1-(3-PYRROLIDIN-1-YLPHENYL)METHANAMINE 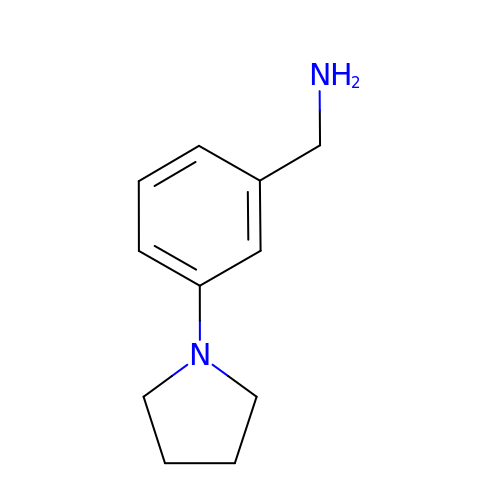| C11 H16 N2 | BXTWTBYGOKOWQX-UHFFFAOYSA-N> MRSRRVDVMDVMNRLILAMDLMNRDDALRVTGEVREYID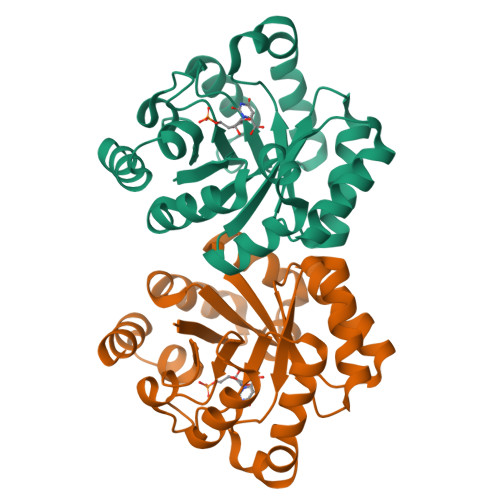TVKIGYPLVLSEGMDIIAEFRKRFGCRIIAAFAVADIPETNEKICRATFKAGADAIIVHGFPGADSVRACLNVAEEMGREVFLLTEMSHPGAEMFIQGAADEIARMGVDLGVKNYVGPSTRPERLSRLREIIGQDSFLISPGVGAQGGDPGETLRFADAIIVGRSIYLADNPAAAAAGIIESIKDLLIPEDPAANKARKEAELAAATA>RERPHTSGHHGAGEARATAPSTVSPYGPEARAELSSRLTTLRNTLAPATNDPRYLQACGGEKLNRFRDIQCRRQTAVRADLNANYIQVGNTRTIACQYPLQSQLESHFRMLAENRTPVLAVLASSSEIANQRFGMPDYFRQSGTYGSITVESKMTQQVGLGDGIMADMYTLTIREAGQKTISVPVVHVGNWPDQTAVSSEVTKALASLVDQTAETKRNMYESKGSSAVADDSKLRPVIHCRAGVGRTAQLIGAMCMNDSRNSQLSVEDMVSQMRVQRNGIMVQ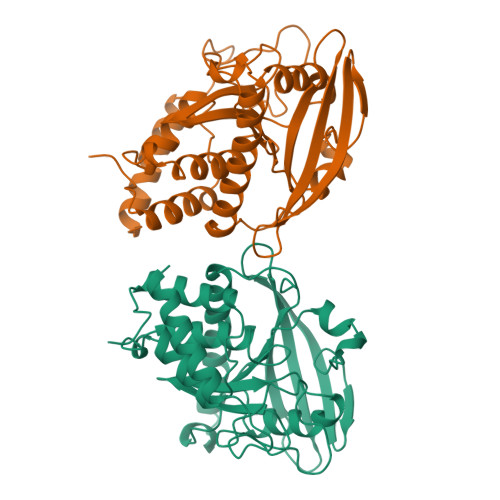KDEQLDVLIKLAEGQGRPLLNS[2x]> XGATQSFQSVGDLTPAEKDLIRSTWDQLMTHRTGFVADVFIRIFHNDPTAQRKFPQMAGLSPAELRTSRQMHAHAIRVSALMTTYIDEMDTEVLPELLATLTRTHDKNHVGKKNYDLFGKVLMEA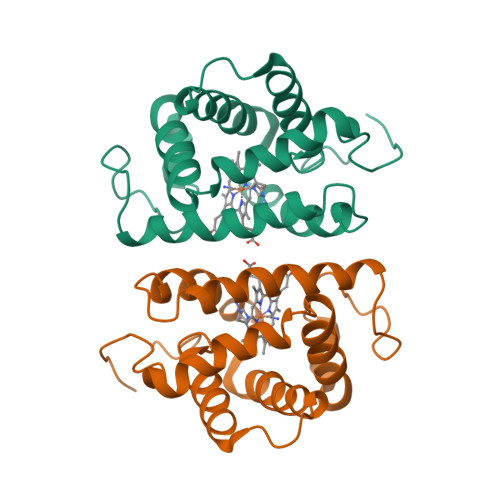IKAELGVGFTKQVHDAWAKTFAIVQGVLITKHAS>[2x]MTREEARRRINELRDLIRYHNYRYYVLADPEISDAEYDRLLRELKELEERFPEFKSPDSPTEQVGARPLEPTFRPVRHPTRMYSLDNAFTYEEVLAFEERLEREAEAPSLYTVEHKVDGLSVLYYEEGVWSTGSGDGEVGEEVTQNLLTIPTIPRRLKGVPDRLEVRGEVYMPIEAFLRLNEELEERGEKVFKNPRNAAAGSLRQKD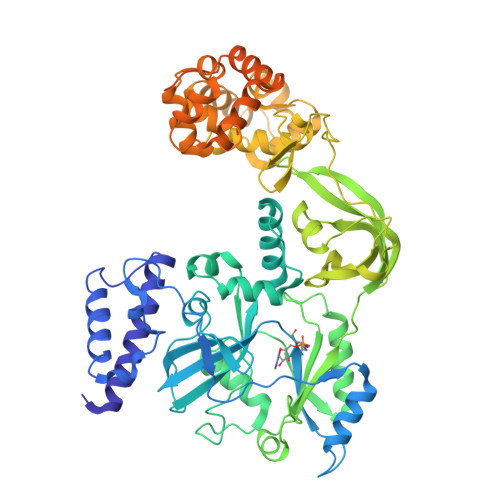PRVTAKRGLRATFYALGLGLGLEESGLKSQYELLLWLKEKGFPVEHCYEKALGAEGVEEVYRRGLAQRHALPFEADGVVLKLDDLTLWGELGYTARAPRFALAYKFPAEEKETRLLDVVFQVGRTGRVTPVGVLEPVFIEGSEVSRVTLHNESYIEELDIRIGDWVLVHKAGGVIPEVLRVLKERRTGKERPIRWPEACPECGHRLVKEGKVHRCPNPLCPAKRFEAIRHYASRKAMDIEGLGEKLIERLLEKGLVRDVADLYHLRKEDLLGLERMGEKSAQNLLRQIEESKHRGLERLLYALGLPGVGEVLARNLARRFGTMDRLLEASLEELIEVEEVGELTARAILETLKDPAFRDLVRRLKEAGVSMESKEEVSDLLSGLTFVLTGELSRPREEVKALLGRLGAKVTDSVSRKTSYLVVGENPGSKLEKARALGVAVLTEEEFWRFLKEKGAPVPA>[2x]ANPNHPLLKKILMKAPGTYHHSMMVANLAEACADKIGANSLLVRVGCFYHDIGKTLRPPYFVENQLQGINPHDRLTPEQSRDIILSHTKDGAEILKENHMPQPIIDIALQHHGTTLLKYF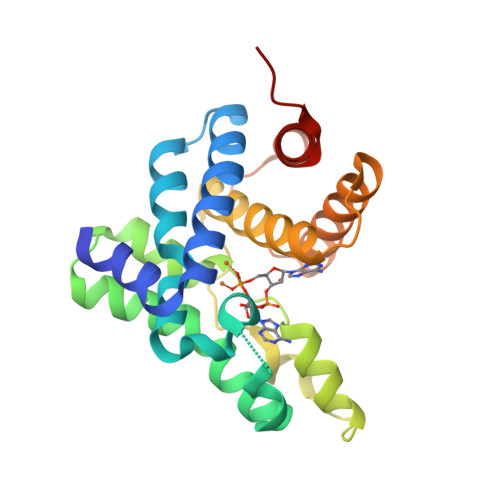YFKAKETNPDVKEADYRYSGPKPQTKEIAIINISDSVEAAVRSSTEPTMAKITEIIDGIIKDRFLDGQFTECDITIQEIKIIRDTLIATLNGIYHQRIQYPD>MVDNSRTRPRVGHIQFLNCLPLYWGLARTGTLLDFELTKDTPEKLSEQLVRGDLDIGPVTLVEFLKNADDLVAFPDIAVGCDGPVMSCVIVSQVPLDRLDGARVALGSTSRTSVRLAQLLLSERFGVQPDYYTCPPDLSLMMQEADAAVLIGDAALRANMIDGPRYGLDVHDLGALWKEWTGLPFVFAVWAARRDYAER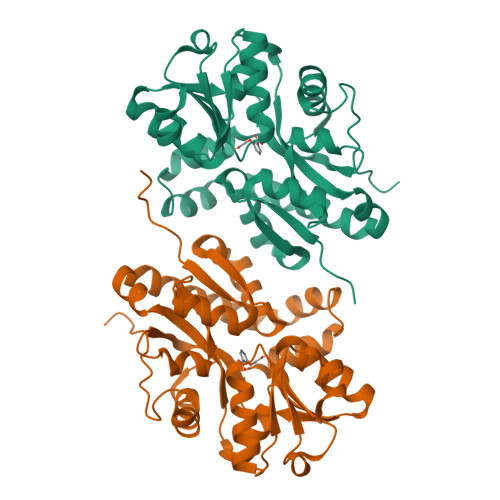EPVITRKVHEAFLASRNLSLEEVEKVAEQAARWEAFDEDTLAKYFTTLDFRFGAPQLEAVTEFARRVGPTTGFPADVKVELLKPLEHHHHHH[2x]> GSMPGFLTAFEYSEKRKMVFHITTGSQEFDKLLGGGIESMAITEAFGEFRTGKTQLSHTLCVTAQLPGAGGYPGGKIIFIDTENTFRPDRLRDIADRFNVDHDAVLDNVLYARAYTSEHQMELLDYVAAKFHEEAGIFKLLIIDSIMALFRVDFSGRGELAERQQKLAQMLSRLQKISEEYNVAVFVTNQMTADPGATMTFQADPKKPIGGHILAHASTTRISLRKGRGELRIAKIYDS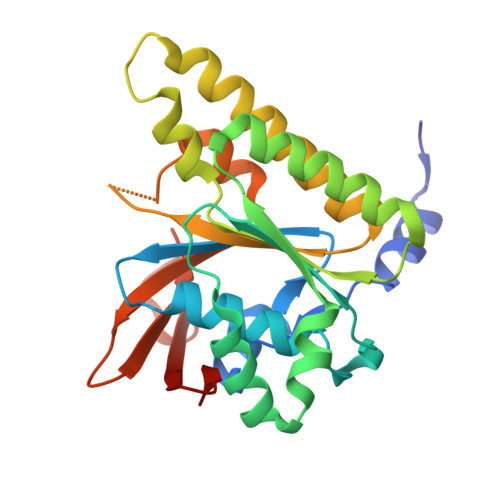PEMPENEATFAITAGGIGDAKE> GSSPVQSGFNNGTISNYMYFERRPDLLTKGTQDKAAAVKLKIENFYQSSVKYAIERNERRVELETELTSHNWSEERKSRQLSSLGKKESQFLRLRRTRLSLEDFHTVKVIGKGAFGEVRLVQKKDTGKIYAMKTLLKSEMYKKDQLAHVKAERDVLAGSDSPWVVSLYYSFQDAQYLYLIMEFLPGGDLMTMLIRWQLFTEDVTRFYMAECILAIETIHKLGFIHRAIKPDNILIDIRGHIKLSDFGLSTGFHKTHDSNYYKKLLQQDEATNGISKPGTYNANTT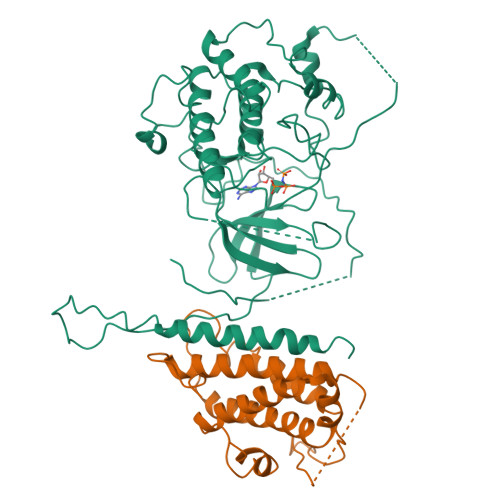DTANKRQTMVVDSISLTMSNRQQIQTWRKSRRLMAYSTVGTPDYIAPEIFLYQGYGQECDWWSLGAIMYECLIGWPPFCSETPQETYRKIMNFEQTLQFPDDIHISYEAEDLIRRLLTHADQRLGRHGGADEIKSHPFFRGVDWNTIRQVEAPYIPKLSSITDTRFFPTDELENVPDSPAMAQAAKQREQMTKQGGSAPVKEDLPFIGYTYSRFDYLTRKNAL;> GSRNKHHSPKRHSQTSFPAQKSTPQSQQLTSTTPQSQQQEASERSESQQIMFLSEPFVRTALVKGSFKTIVQLPKYVDLGEWIALNVFEFFTNLNQFYGVVAEYVTPDAYPTMNAGPHTDYLWLDANNRQVSLPASQYIDLALTWINNKVNDKNLFPTKNGLPFPQQFSRDVQRIMVQMFRIFAHIYHHHFDKIVHLSLEAHWNSFFSHFISFAKEFKIIDRKEMAPLLPLIESFEKQGKIIYN> MSLRRGIYHIENAGVPSAIDLKDGSSSDGTPIVGWQFTPDTINWHQLWLAEPIPNVADTFTLCNLFSGTYMDLYNGSSEAGTAVNGWQGTAFTTNPHQLWTIKKSSDGTSYKIQNYGSKTFVDLVNGDSSDGAKIAGWTGTWDEGNPHQKWYFNRMSVSSAEAQAAIARNPHIHGTYRGYILDGEYLVLPNATFT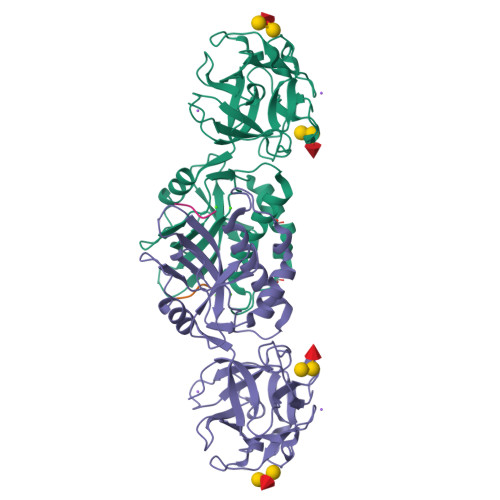QIWKDSGLPGSKWREQIYDADDFAIAMKAAVGKWGADSWKANGFAIFCGVMLGVNKAGDAAHAYNFTLTKDHADIVFFEPQNGGYLNDIGYDSYMAFY;> PVPR>[4x]MGSSHHHHHHSSGENLYFQGHMSNTSWRKSEVLAVPLQPTLQQEVILARMEQILASRALTDDERAQLLYERGVLYDSLGLRALARNDFSQALAIRPDMPEVFNYLGIYLTQAGNFDAAYEAFDSVLELDPTYNYAHLNRGIALYYGGRDKLAQDDLLAFYQDDPNDPFRSLWLYLAEQKLDEKQAKEVLKQHFEKSDKEQWGWNIVEFYLGNISEQTLMERLKADATDNTSLAEHLSETNFYLGKYYLSLGDLDSATALFKLAVANNVHNFVEHRYALLELSLLGQDQDDLAESDQQ;>MSANNTAKNMHPETRAVGSETSSLQASQDEFENLVRNVDVKSRIMDQYADWKGVRYRLGGSTKKGIDCSGFVQRTFREQFGLELPRSTYEQQEMGKSVSRSNLRTGDLVLFRAGSTGRHVGIYIGNNQFVHASTSSGVIISSMNEPYWKKRYNEARRVLSRSHHHHHH[8x]

During cell growth, PG endopeptidases cleave the crosslinks of the fully closed sacculi, allowing for the incorporation of new glycan strands and expansion of the peptidoglycan mesh. Outer-membrane-anchored NlpI associates with hydrolases and synthases near PG synthesis complexes, facilitating spatially close PG hydrolysis. The protein level of MepS is known to be regulated by the periplasmic PDZ-protease Prc (or tsp, tail-specific protease) in complex with the adaptor NlpI42. The structure of NlpI in complex with MepS provides molecular insight into NlpI-interacting endopeptidase colocalization, while the Prc-NlpI-MepS complex elucidates the molecular mechanism of NlpI-mediated MepS degradation by the tail-specific protease Prc.

To characterize the basis of how the lipoprotein NlpI mediated the endopeptidase colocalization near the outer membrane, we determined a 2.8 Å resolution structure of NlpI in complex with mMepS by X-ray crystallography. The structure revealed a heterohexameric complex with a homodimer of NlpI bound to four mMepS molecules. Moreover, the SAXS profile of NlpI-mMepS is consistent with the crystallographic results, with χ2 = 1.73, confirming that the hexameric structure does exist in solution. Surprisingly, the intrinsically disordered N-terminal of monomeric mMepS becomes folded and dimerized upon NlpI binding, thereby guiding four mMepS to form two asymmetric dimers bound to a homodimeric NlpI (namely NlpI and NlpI’). One protomer (mMepS-1) of NlpI-bound mMepS has the extended α1 (residues Q28 to W51), while the 12-residue segment comprising Q28 to D39 lacks a defined secondary structure in its apo state. This segment simultaneously engages in extensive interactions with the h1 of NlpI and the h3’ of NlpI’ located at the dimerization interface of NlpI, thus contributing to the extension of α1 by approximate 3.3 turns and 18 Å. The core structure of mMepS-1 mainly interacts with that of mMepS-2, while the extended α1 of mMepS-1 engages the interface of NlpI dimer. Notably, mMepS-2 of the complex structure simultaneously engages mMepS-1 and one protomer NlpI but not the other NlpI’. We conclude that the colocalization of four mMepS molecules can be mediated by a NlpI homodimer, suggesting that multiple mMepS may work cooperatively and thus enhance the avidity of mMepS-PG interaction.> GPGSMDALVDY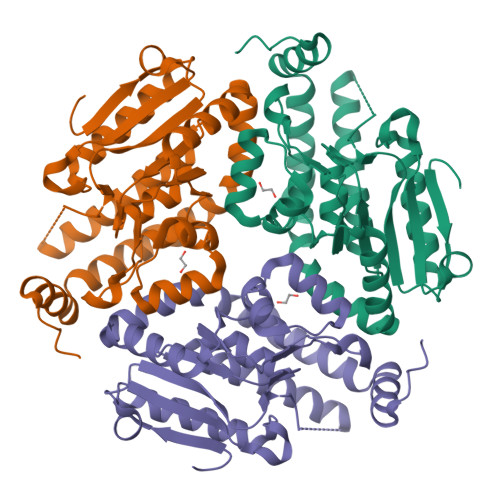AGPAATGGPVARLTLNSPHNRNALSTALVSQLHQGLRDASSDPAVRVVVLAHTGGTFCAGADLSEAGSGGSPSSAYDMAVERAREMAALMRAIVESRLPVIAAIDGHVRAGGFGLVGACDIAVAGPRSSFALTEARIGVAPAIISLTLLPKLSARAAARYYLTGEKFDARRAEEIGLITMAAEDLDAAIDQLVTDVGRGSPQGLAASKALTTAAVLERFDRDAERLAEESARLFVSDEAREGMLAFLEKRSPNWTS Vibrio cholerae contains multiple copies of chemotaxis response regulator (VcCheY1–VcCheY4) whose functions are elusive yet. Autophosphorylated CheA then donates phosphate to the response regulator CheY. Phosphorylated CheY interacts with the flagellar motor protein FliM and influence the direction of flagellar rotation from counter clock wise (CCW) to clock wise (CW). As expected, both VcCheY3 and VcCheY4 possess (β/α)5 fold typical of the response regulators.

We have solved the structures of VcCheY3 in Ca2+ and Mg2+ bound states to the resolutions of 1.67 Å and 2.2 Å respectively. The location of the Ca2+ (or Mg2+) ion in VcCheY3 is similar to that of Mg2+ ion in StCheY. The Ca2+ (or Mg2+) of VcCheY3 is heptacoordinated where four coordinations occur with protein atoms and three with water molecules. Although D12 of StCheY is not coordinated to Mg2+, D15 of VcCheY3 that corresponds to D12 of StCheY, coordinates with the metal ion. The average coordination distance between Ca2+ and the protein atoms is about 2.4 Å while this is of about 2.1 Å in case of Mg2+ which is due to the size difference of the ions. D60 is the site of phosphorylation in VcCheY3 as it corresponds to D57 of StCheY. Both in the Mg2+ and Ca2+ bound free state structures of VcCheY3, the side chain of W61 (that corresponds to W58 of StCheY) is observed in a conformation, substantially different from that of StCheY. From the crystal structures of Ca2+ and Mg2+ bound VcCheY3 we proposed the presence of a conformational barrier composed of the hydrophobic packing of W61, M88 and V106 and a unique hydrogen bond between T90 and Q97 in VcCheY3.

> ANKNMKILIVDDFSTMRRIVKNLLRDLGFNNTQEADDGLTALPMLKKGDFDFVVTDWNMPGMQGIDLLKNIRADEELKHLPVLMITAEAKREQIIEAAQAGVNGYIVKPFTAATLKEKLDKIFE>[4x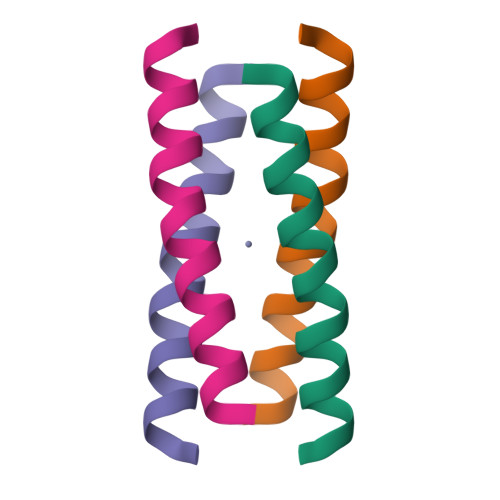]XIEELLRKIIEDEVRHIAELEDIEKWLX>MGSDKIHHHHHHMRVELLFESGKCVIDLNEEYEVVKLLKEKI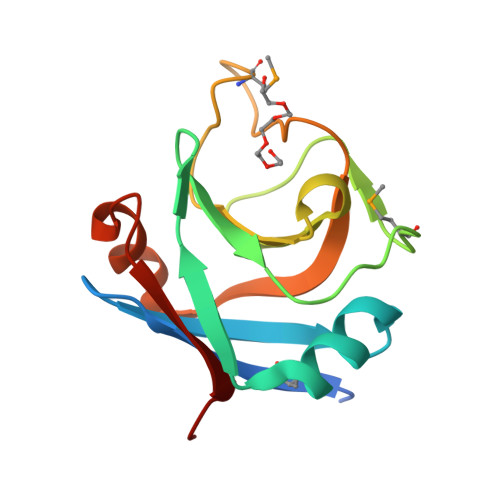PFESVVNTWGEEIYFSTPVNVQKMENPREVVEIGDVGYWPPGKALCLFFGKTPMSDDKIQPASAVNVIGKIVEGLEDLKKIKDGEKVAVRFASS[3x]> MGEKQEEEGEEEKEGKGEGGGEGGREEEDEDGSAPVVSWLRIVEERECHEETDEAPETKIALPFSAQRSSRGFEARQVEVLVSANSAFLLSVLLASLFLSSSLPSFCPPRFLLSVLLALFKDKMAGDAPAAAAAPQQAGRTASASGVRTPGYLDLVGHSLK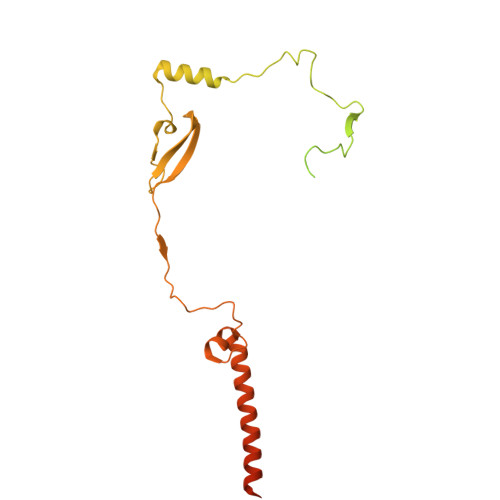ATSMDHGMQYSSIYWETSHRTYLPFWASLTQKFSWKIMDDQIRSFLRLPKPVTTEPFVFSSGSPYIRRYFGDADISVPVPLHAPAHFAFVPTGTVSPWEETGMETGPQGAAARGAAATAFRAVLESAWKCDIDEQIKEKLHSRAGAGAFHASGSTGGCPIPTDF>GGCGGCGGCGGCUGCUGCC[2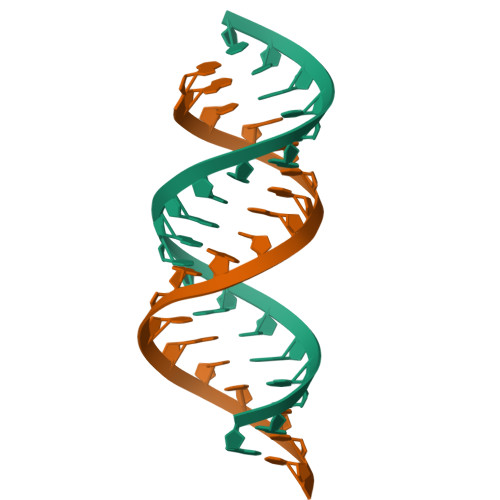x]>[2x]MYLIEPKRNGKWVFDGAILLAIQYWAIKNLKLDETIVFPYICDPHVQIGYFQNPSVEVNLELLKQKNIEVVRRDTGGGAIYLDRNGVNFCFSF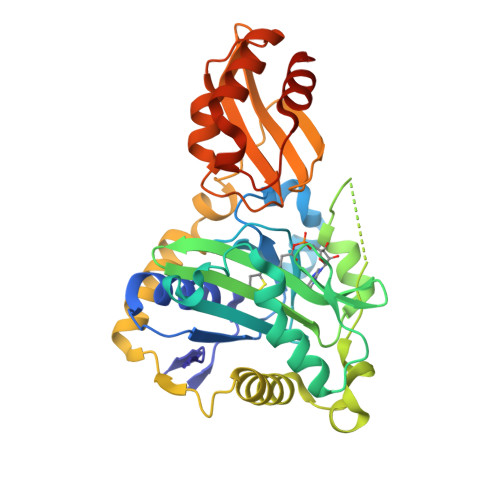PYEKNKNLLGNYAQFYDPVIKVLQNIGIKNVQFSGKNDLQIEGKKVSGAAMSLVNDRIYAGFSLLYDVDFDFIGKILTPNQKKIEAKGIKSVSQRVTNLKNKLSKEYQNFSIFEIKDLFLTEFLKVNSVEKFKKYELTDSDWVQIDKMVAEKYKNWDFVWGLSPNYSFNRSIRTKVGTITFSLEINEGKISKIKISGDFFPKKSLLELENFLMGTKLTQDQLLNRLKDAKLEDYFSQKIDEEEICNLLLNLEHHHHHH> GLECDGKVNICCKKQFFVSFKDIGWNDWIIAPSGYHANYCEGECPSHIAGT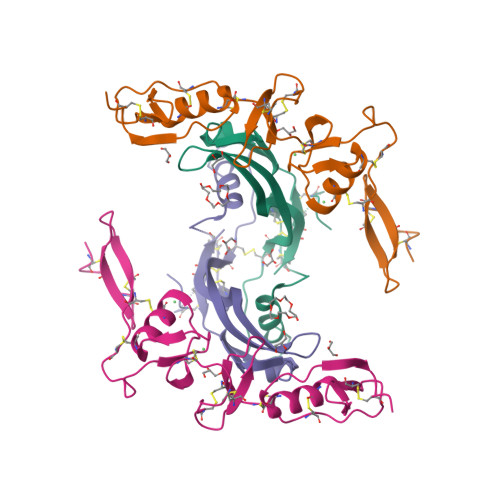SGSSLSFHSTVINHYRMRGHSPFANLKSCCVPTKLRPMSMLYYDDGQNIIKKDIQNMIVEECGCS;> GSMETCENVDCGPGKKCRMNKKNKPRCVCAPDCSNITWKGPVCGLDGKTYRNECALLKARCKEQPELEVQYQGKCKKTCRDVFCPGSSTCVVDQTNNAYCVTCNRICPEPSSSEQSLCGNDGVTYSSACHLRKATCLLGRSIGLAYEGKCIK Here, we chose aminodeoxychorismate synthase (ADCS) from Escherichia coli, which consists of a class I glutaminase subunit (PabA) and a synthase subunit (PabB), to investigate the mechanism of glutaminase catalysis regulation and its impact on overall GAT activity. PabB catalyzes the amination of chorismate (Cho) to 4-amino-4-deoxy-chorismate, which is a committed step in folic acid biosynthesis. GATs comprise minimally a glutaminase that produces ammonia, which reacts with a synthase-bound substrate to yield specific nitrogen-containing products. As evidenced by analytical gel filtration and isothermal titration calorimetry (ITC) data, the PabA and PabB subunits form a heterodimeric assembly with a dissociation constant KD = 0.16 ± 0.06 μM.

Finally, we assessed whether a catalytically competent conformation of the glutaminase active site requires rigidification by the presence of the synthase subunit PabB, by determining an additional crystal structure of the separate PabA subunit. Indeed, a comparison of these structures reveals a significant increase in ordering of the glutaminase active site in the presence of PabB due to reduced conformational variability of several interface PabA loops, which is required to generate a catalytically competent arrangement of the two catalytic triad residues aH168 and aE170. While we found only residual glutaminase activity in separate PabA, the catalytic glutaminase efficiency kcat/KMGln of the ADCS complex in the presence of Mg2+ and Cho was 1.09 ± 0.13 mM−1s−1, which is similar to previously reported data.

>[3x]GGMILLIDNYDSFTWNLYQYFCELGADVLVKRNDALTLADIDALKPQKIVISPGPCTPDEAGISLDVIRHYAGRLPILGVCLGHQAMAQAFGGKVVRAAKVMHGKTSPITHNGEGVFRGLANPLTVTRYHSLVVEPDSLPACFDVTAWSETREIMGIRHRQWDLEGVQFHPESILSEQGHQLLANFLHR>GHMPLLSASIVSAPVVTSETYVDIPGLYLDVAKAGIRDGKLQVILNVPTPYATGNNFPGIYFAIATNQGVVADGCFTYSSKVPESTGRMPFTLVATIDVGSGVTFVKGQWKSVRGSAMHIDSYASLSAIWGTAA[3x]

The bacterial lectin BC2L‐C expressed in B. cenocepacia is an interesting drug target involved in bacterial adhesion and subsequent deadly infection to the host. For BC2L‐C, the C‐terminal domain (LecB like) specifically binds to mannose, while the N‐terminal domain (BC2L‐C‐nt) has been structurally characterized as a novel fucose‐binding domain with a trimeric TNF‐α‐like architecture. Thus, BC2L‐C represents a novel type of superlectin with dual specificity for fucose and mannose in the N‐ and C‐terminal domains, respectively. BC2L‐C as a virulence factor binds to carbohydrates present on the epithelial cells of the host.

Crystal structure analysis of the apo and the holo form of BC2L‐C‐nt demonstrated the presence of a druggable (ligandable) region (site X) in the vicinity of the fucoside binding site. Of the two other regions (X and Z), site X is a deep crevice extending along the binding interface. The study indicates that the fragments bind in a newly identified binding region in BC2L‐C‐nt when the fucoside binding site is occupied. Remarkably, the binding mode of one fragment (KL3) could be validated by X‐ray crystallography at high resolution, further confirming the ability of site X to host drug‐like fragments. ITC and X‐ray crystallography performed on one fragment confirmed binding at the expected location and therefore the ability of site X to host drug‐like fragments. The affinity measured by ITC is sub‐millimolar, which is very promising for such small fragment. The complementary structural and thermodynamic data give clear view of the relative importance of apolar and polar interactions for fragment KL3. This could be used in the future for structure‐based optimization of this first hit. The selection of suitable linkers can be done based on the distance (measured 4.8 Å) between the nearest atoms of fragment and the fucose core.>MSKSDVFHLGLTKNDLQGAQLAIVPGDPERVEKIAALMDKPVKLASHREFTSWRAELDGKAVIVCSTGIGGPSTSIAVEELAQLGIRTFLRIGTT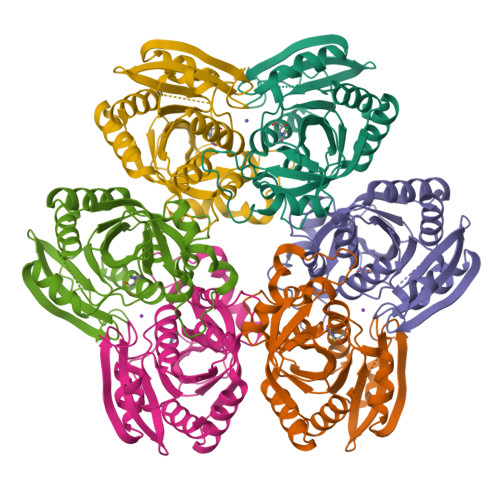GAIQPHINVGDVLVTTASVRLDGASLHFAPMEFPAVADFACTTALVEAAKSIGATTHVGVTASSDTFYPGQERYDTYSGRVVRRFKGSMEEWQAMGVMNYEMESATLLTMCASQGLRAGMVAGVIVNRTQQEIPNAETMKQTESHAVKIVVEAARRLL[9x]S-layer proteins (SLPs) are self-assembling, crystalline proteins coating the cell surfaces of many prokaryotes. We determined the atomic resolution structures of all functional domains (I-III from N- to C-termini) present in the three S-layer proteins SlpA_ac, SlpX_ac, and SlpA_amy. The Lactobacillus S-layers are anchored to the cell wall through interaction with teichoic acids (TA), either lipoteichoic acid (LTA) or wall teichoic acid (WTA).

The SlpA protein (~46 kDa) is the main structural component of Lactobacillus acidophilus ATCC 4356 S-layer, built of two domains. The N-terminal region is involved in the self-assembly of the S-layer, whereas the C-terminal part is involved in the attachment to the cell wall. The amino acid sequence of the C-terminal SlpA_III domain is sequentially conserved among Lactobacillus. It consists of two adjacent repeats of the “SlpA-motif,” the “Surface layer protein A motif/domain” (InterPro: IPR024968). This domain is involved in the binding to TAs (teichoic acid binding domain; TAB domain), one of the components of the bacterial cell wall. The crystal structures of the TAB domains (SlpA_ac_III, SlpA_amy_III, and SlpX_ac_III) reveal high structural similarities. The general structure of the TAB domain consists of two cell wall binding motifs (SlpA_motif) which are connected by a short linker and arranged as an internal homodimer. Mapping of the surface charges indicates a large, highly positively charged region within the interface of the two motifs that extends to the C-terminal part of the protein. The four residues observed in the vicinity of phosphates are conserved with the proposed binding motif of YxY….KxxN. SlpA_III, the teichoic acid binding domain, is not involved in the self-assembly and protrudes inward to the bacterial cell.

> VASVSKRIMHNAYYYDKDAKRVGTDSVKRYNSVSVLPNTTTINGKTYYQVVENGKAVDKYINAANIDGTKRTLKHNAYVYASSKKRANKVVLKKGEVVTTYGASYTFKNGQKYYKIGDNTDKTYVKVANFR>[2x]GGGSMEPGRGGTETVGKFEFSRKDLIGHGAFAVVFKGRHRAAHDLEVAVKCINKKNLAKSQTLLGKEIKILKELKHENIVALYDFQEMANSVYLVMEYCNG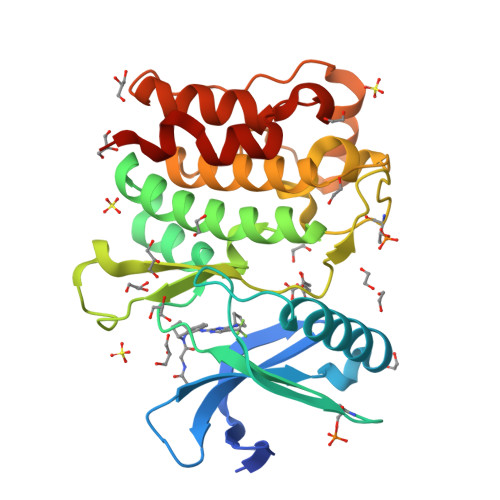GDLADYLHAMRTLSEDTIRLFLQQIAGAMRLLHSKGIIHRDLKPQNILLSNPAGRRANPNSIRVKIADFGFARYLQSNMMAATLCGSPMYMAPEVIMSQHYDGKADLWSIGTIVYQCLTGKAPFQASSPQDLRLFYEKNKTLVPTIPRETSAPLRQLLLALLQRNHKDRMDFDEFFHHPFLDASPS>MRGSFANDATFEIKKCDLHRLEEGPPVTTVLTREDGLKYYRMMQTVRRMELKADQLYKQKIIRGFCHLCDGQEACCVGLEAGINPTDHLITAYRAHGFTFTRGLSVREILAELTGRKGGCAKGKGGSMHMYAKNFYGGNGIVGAQVPLGAGIALACKYNGKDEVCLTLYGDGAANQGQIFEAYNMAALWKLPCIFICENNRYGMGTSVERAAASTDYYKRGDFIPGLRVDGMDILCVREATRFAAAYCRSGKGPILMELQTYRYHGHSMSDPGVSYRTREEIQEVRSKSDPIMLLKDRMVNSNLASVEELKEIDVEVRKEIEDAAQFATADPEPPLEELGYHIYSSDPPFEVRGANQWIKFKSVS[2x];>[2x]MRGSHHHHHHGSLQVTVRDAINQGMDEELERDEKVFLLGEEVAQYDGAYKVSRGLWKKYGDKRIIDTPISEMGFAGIAVGAAMAGLRPICEFMTFNFSMQAIDQVINSAAKTYYMSGGLQPVPIVFRGPNGASAGVAAQHSQCFAAWYGHCPGLKVVSPWNSEDAKGLIKSAIRDNNPVVVLENELMYGVPFEFPPEAQSKDFLIPIGKAKIERQGTHITVVSHSRPVGHCLEAAAVLSKEGVECEVINMRTIRPMDMETIEASVMKTNHLVTVEGGWPQFGVGAEICA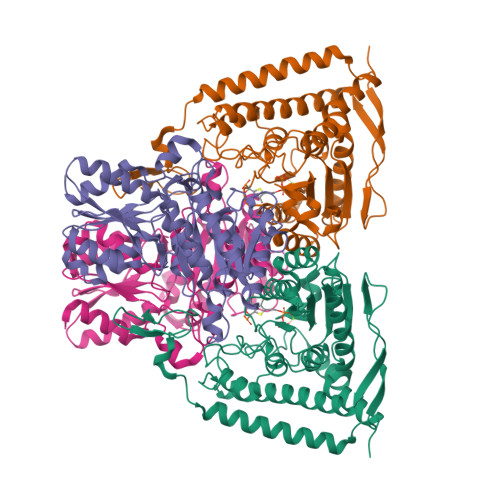RIMEGPAFNFLDAPAVRVTGADVPMPYAKILEDNSIPQVKDIIFAIKKTLNI> MNGWNFQELKETPSQTGGPYVHIGLLPKQANIEVFEHNLDNNLVQDNTQGQRIRLEGQVFDGLGLPLRDVLIEIWQADTNGVYPSQADTQGKQVDPNFLGWGRTGADFGTGFWSFNTIKPGAVPGRKGSTQAPHISLIIFARGINIGLHTRVYFDDEAEANAKDPVLNSIEWATRRQTLVAKREERDGEVVYRFDIRIQGENETVFFDI;> MSQIIWGAYAQRNTEDHPPAYAPGYKTSVLRSPKNALISIAETLSEVTAPHFSADKFGPKDNDLILNYAKDGLPIGERVIVHGYVRDQFGRPVKNALVEVWQANASGRYRHPNDQYIGAMDPNFGGCGRMLTDDNGYYVFRTIKPGPYPWRNRINEWRPAHIHFSLIADGWAQRLISQFYFEGDTLIDSCP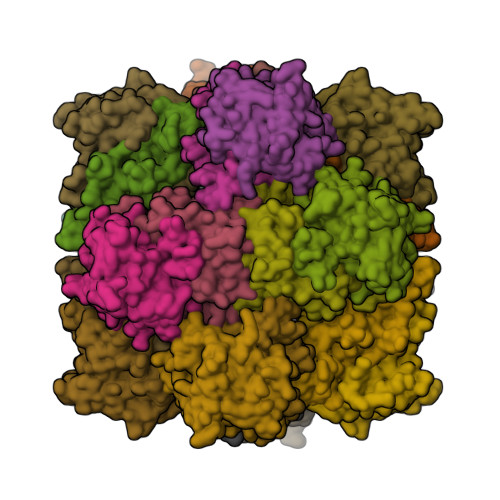ILKTIPSEQQRRALIALEDKSNFIEADSRCYRFDITLRGRRATYFENDLT> MSLSDDIKVLGISGSLRSGSYNSAALQEAIGLVPPG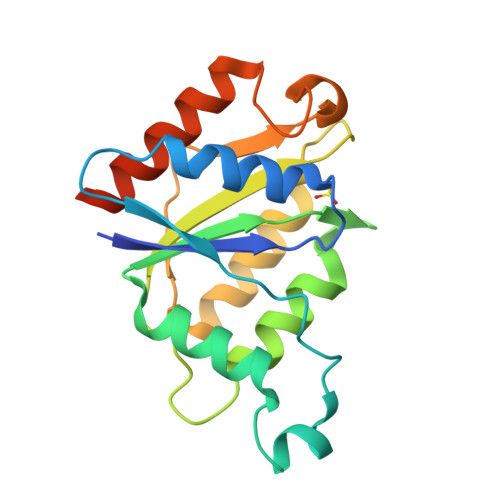MSIELADISGIPLYNEDVYALGFPPAVERFREQIRAADALLFATPEYNYSMAGVLKNAIDWASRPPEQPFSGKPAAILGASAGRFGTARAQYHLRQTLVFLDVHPLNKPEVMISSAQNAFDAQGRLLDDKARELIQQQLQALQLWVREGGSHHHHHH> GPKHDGRVKIGHYVLGDTLGVGTFGKVKIGEHQLTGHKVAVKILNRQKIRSLDVVGKIKREIQNLKLFRHPHIIKLYQVISTPTDFFMVMEYVSGGELFDYICKHGRVEEMEARRLFQQILSAVDYCHRHMVVHRDLKPE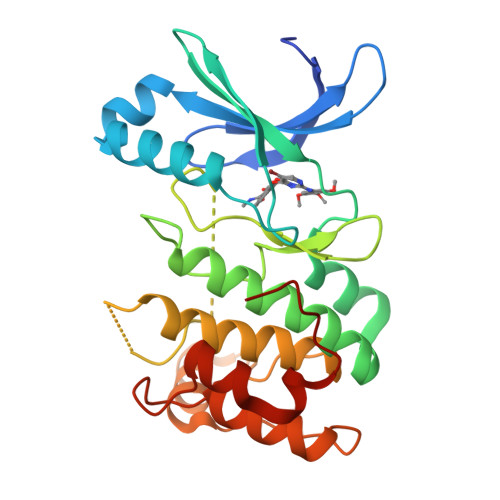NVLLDAHMNAKIADFGLSNMMSDGEFLRDSCGSPNYAAPEVISGRLYAGPEVDIWSCGVILYALLCGTLPFDDEHVPTLFKKIRGGVFYIPEYLNRSVATLLMHMLQVDPLKRATIKDIREHEWFKQDLPSYLFPE>[2x]MKILKDDAPELHAIAAEVPHGEDVKDLVLDMTAAMTAAGGIGLAG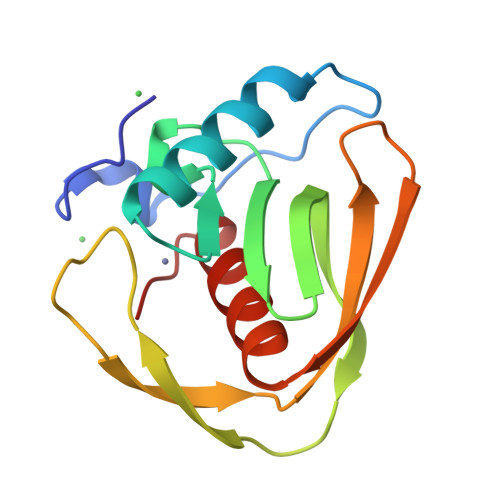NQVGVLKRIIVLRCPTFKGCVINPIITRHTDGHVYSPEGCLSYPGKTVAKKRRNKVVVEGYDMDWQPITIAAKGLTAFCLQHEIDHLNGVTI> MGKVSTPKVHVYSHFPGEYGKPNTLICYVSSFHPPDISIELLKNGQVMSDTKQTDLAFEKGWQFHLTKSVAF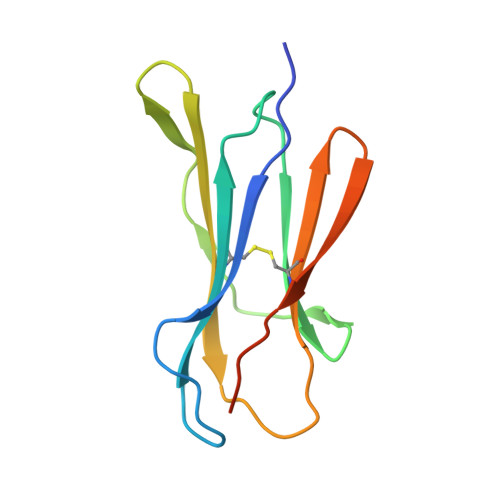TPEKGDEYTCSVRHMKETKKFSWEPNMLEHHHHHH> KKPEIAQVIASYTATGPEQLTLAPGQLILIRKKNPGGWWEGE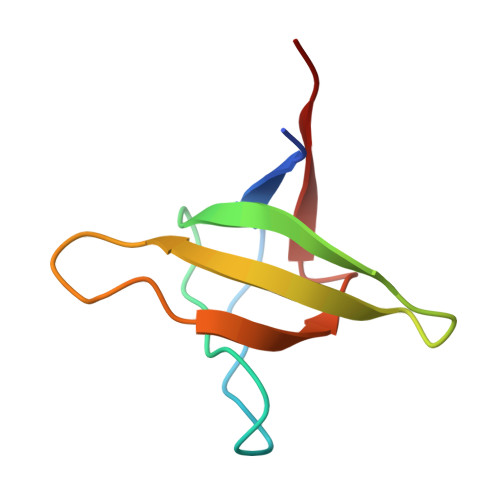LQARGKKRQIGWFPANYVKLLSP In this work, a BGL from the thermophilic and halophilic bacterium Halothermothrix orenii, HoBGLA, was characterized biochemically and structurally. It is an unspecific β-glucosidase with mixed activities for different substrates and prominent activity with various galactosidases such as lactose. The overall structure of the 451-residue large HoBGLA displays the typical (β/α)8 TIM-barrel fold adopted by retaining GH1 enzymes. In subsite −1 of the active site, the catalytic residues Glu354 (nucleophile) and Glu166 (acid/base catalyst) are situated near Glu408.

The 2.0 Å structure of the 2-deoxy-2-fluoroglucopyranosyl-HoBGLA intermediate was obtained by soaking crystals with only 2FGlc and not with an activated compound such as 2,4-dinitrophenyl 2-deoxy-2-fluoro-β-d-glucoside (DNP-2FGlc) or 2-deoxy-2-fluoro-β-d-glucosyl fluoride. Nonetheless, the catalytic nucleophile appears to be labeled by 2FGlc in both molecules of the asymmetric unit with covalent-bond (Glu354 Oε1–2FGlc C1) distances of 1.60 and 1.58 Å, respectively. It is likely that the covalent complex is a result of reverse hydrolysis. Based on the elongated bond distance compared with that expected for a stable covalent intermediate (about 1.35 to 1.45 Å), the structure may reflect a somewhat destabilized covalent complex. However, there are no obvious alternative orientations of either the 2FGlc molecule or the Glu354 side chain. It is also clear from the electron density that the equatorial O1 hydroxyl group for 2FGlc has been removed. The Glu408 Oε1 and Oε2 oxygen atoms participate in substrate binding by offering two hydrogen bonds to O4 in 2FGlc. Trp401 provide hydrophobic stacking with the glucosyl residue in this subsite and additional protein-sugar hydrogen bonds are formed by Gln20, Trp409, His121, Asn165, and Glu354. The puckering parameters [φ = 103.4°, θ = 7.0°, Q = 0.64] are consistent with a 4 C 1 chair with a slight distortion in the direction of a 2,5 B boat/5 S 1 skew boat. The attachment of an electronegative fluorine atom close to the reacting carbon atom serves to destabilize the oxocarbenium ion-like transition state and reduces the reaction rates in both the glycosylation and deglycosylation steps of the retaining reaction.

>SMAKIIFPEDFIWGAATSSYQIEGAFNEDGKGESIWDRFSHTPGKIENGDTGDIACDHYHLYREDIELMKEIGIRSYRFSTSWPRILPEGKGRVNQKGLDFYKRLVDNLLKANIRPMITLYHWDLPQALQDKGGWTNRDTAKYFAEYARLMFEEFNGLVDLWVTHNEPWVVAFEGHAFGNHAPGTKDFKTALQVAHHLLLSHGMAVDIFREEDLPGEIGITLNLTPAYPAGDSEKDVKAASLLDDYINAWFLSPVFKGSYPEELHHIYEQNLGAFTTQPGDMDIISRDIDFLGINYYSRMVVRHKPGDNLFNAEVVKMEDRPSTEMGWEIYPQGLYDILVRVNKEYTDKPLYITENGAAFDDKLTEEGKIHDEKRINYLGDHFKQAYKALKDGVPLRGYYVWSLMDNFEWAYGYSKRFGLIYVDYENGNRRFLKDSALWYREVIEKGQVEAN[2x]>GPLGSPEFMEVICKHYTPLDIASQAIRTCWQSFEYSDDGGCKDKELIHRVGNIFRHSSTLEHLYYNFEIKGLSRGALQELSRHRIASLSVKSSRYTLRELKEVESFLPLNETNLERAREFLVFVDNEKVNAMSVLALENLRVLLSEHNIKNDLAKYAMPESYKTHLAYSINARSLQNLLTLRSSNKALKEMQDLAKALFDALP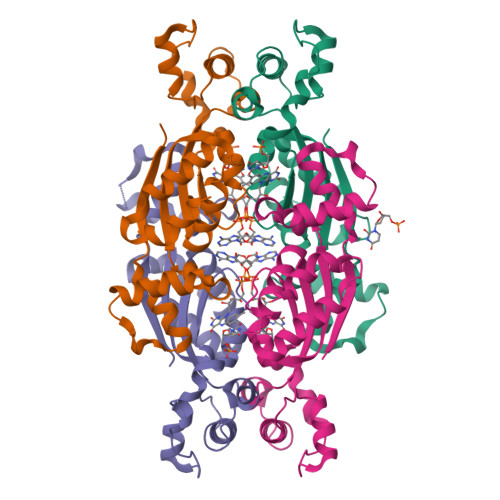GEHQYLFEDCLKH[4x]>[8x]GSEELLDLFNRQVTQEFTASQVYLSASIWFDQNDWEGMAAYMLAESAEEREHGLGFVDFANKRNIPIELQAVPAPVSCAEWSSPEDVWQSILELEQANTRSLLNLAEAASTCHDFAVMAFLNPFHLQQVNEEDKIGSILAKVTDENRTPGLLRSLDVVSFLGPCLFRS

A novel ferritin was recently found in Pseudo-nitzschia multiseries (PmFTN), a marine pennate diatom that plays a major role in global primary production and carbon sequestration into the deep ocean. Ferritin is a 24-mer that forms a hollow sphere, takes up soluble ferrous iron, oxidizes it at di-iron ferroxidase centers, and stores the iron oxide mineral in its central cavity. Sites A and B comprise the conserved ferroxidase active site, and site C forms a pathway leading toward the central cavity where iron storage occurs. The structures confirm the typical ferritin arrangement: 24 subunits assemble to form a hollow spherical shell.

To determine whether occupation of ferroxidase sites and site C is time-dependent, apo-PmFTN crystals were soaked for 5 min, 45 min, 4 h, and overnight in 2 mm ferrous sulfate. Structures of crystals exposed to ferrous iron for 4 h or longer revealed iron bound in all three sites as well as up to two additional sites at the inner surface of the ferritin sphere. The latter two sites may serve as the nucleation site for formation of the mineral core. The iron in site A is coordinated by the conserved residues Glu-15, Glu-48, and His-51. Coordination of the iron bound in site B is by 2–3 glutamate residues, depending on the subunit. A bridging oxygen atom is modeled between sites A and B and between sites B and C. In addition to Glu-130, the site C iron is coordinated by Glu-47 and Glu-44. Glu-130 adopts multiple conformations depending on the soaking time and is observed coordinated to iron atoms in site B and/or site C. In the overnight-soaked structure, Glu-130 is tilted toward the iron in site B, whereas in the 4-h-soaked structure, it is predominately coordinated to site C. Only in crystals incubated in ferrous iron for 4 h and longer was iron bound to site C. In the subunits with water bound to site C, the side chain of Glu-130 adopts an alternative rotamer such that it is directed away from the site and toward the core. In the PmFTN structure soaked aerobically for more than 4 h, Glu-130 is a ligand to iron atoms in sites B and C. In contrast, in the earlier PmFTN structure soaked in iron for 10 min by Marchetti et al., the iron in site C is coordinated by only Glu-44.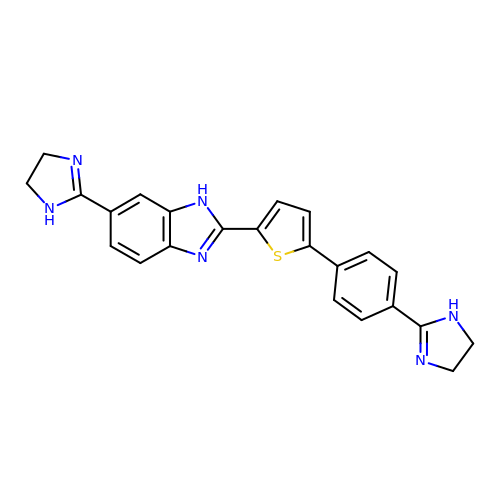6-(4,5-DIHYDRO-1H-IMIDAZOL-2-YL)-2-{5-[4-(4,5-DIHYDRO-1H-IMIDAZOL-2-YL)PHENYL]THIEN-2-YL}-1H-BENZIMIDAZOLE | C23 H20 N6 S | KPAUDMFCLSTUBG-UHFFFAOYSA-N>[4x]MRGSHHHHHHGSMVVKVGVIGTGAMGRAHIDRLTNVLTGAEVVAVTDIDHEAAEAAVRDFHLNAKVYPDDTSLLQDPDIDAVFVVSFGGAHEATVLKALDTDKFIFTEKPLATTLEGAKRIVDKELTKSKKVIQVGFMRRYDQGIRALKEKLDTGIIGAPLVVRASHINPNVASNYSNEMAITDTLIHEIDEMHWLLDDEYTSIQITYPRQSAEVRNEGLHDPQLATLTTKKGTVIQVLVHVT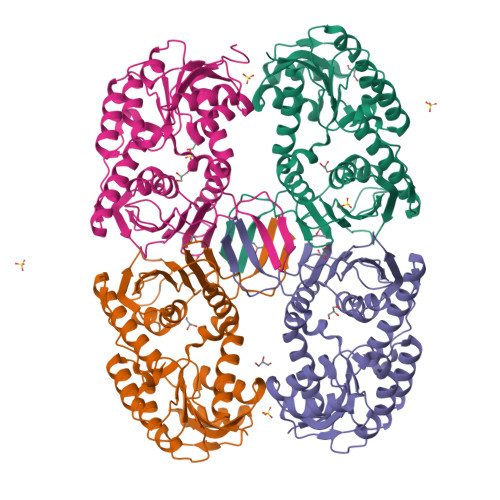AQYGYEVKLEVIGETGELQLPNYGLGPILRSNANQQTAVEMSWINRFIQAYNTEVQEFIDEVAKSEPPVGPSAWDGYIAAITAAAANRSQKDQETVLINVAGTPTFYQ>LPSTKPQLSEEQAAVLRAVLKGQSIFFTGSAGTGKSYLLKRILGSLPPTGTVATASTGVAACHIGGTTLHAFAGIGSGQAPLAQCVALAQRPGVRQGWLNCQRLVIDEISMVEADLFDKLEAVARAVRQQNKPFGGIQLIICGDFLQLPPVTKGSQPPRFCFQSKSWKRCVPVTLELTKVWRQADQTFISLLQAVRLGRCSDEVTRQLQATASHKVGRDGIVATRLCTHQDDVALTNERRLQELPGKVHRFEAMDSNPELASTLDAQCPVSQLLQLKLGA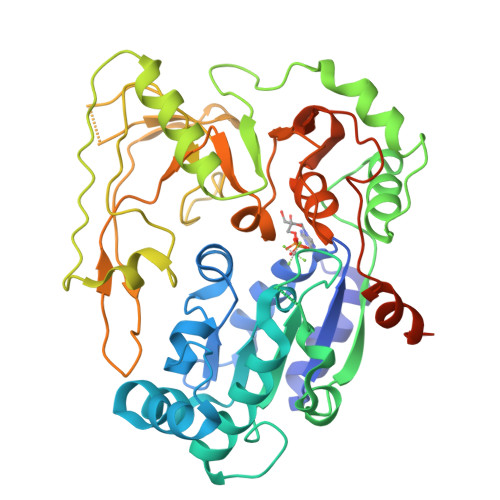QVMLVKNLSVSRGLVNGARGVVVGFEAEGRGLPQVRFLCGVTEVIHADRWTVQATGGQLLSRQQLPLQLAWAMSIHKSQGMTLDCVEISLGRVFASGQAYVALSRARSLQGLRVLDFDPMAVRCDPRVLHFYATLRRGRSLSLESPDDDEAASDQENMDPIL[2x]>[3x]SKKLLFQFDTDATPSVFDVVVGYDGGADHITGYGNVTPDNVGAYVDGTIYTRGGKEKQSTAIFVGGGDMAAGERVFEAVKKRFFGPFRVSCMLDSNGSNTTAAAGVALVVKAAGGSVKGKKAVVLAGTGPVGMRSAALLAGEGAEVVLCGRKLDKAQAAADSVNKRFKVNVTAAETADDASRAEAVKGAHFVFTAGAI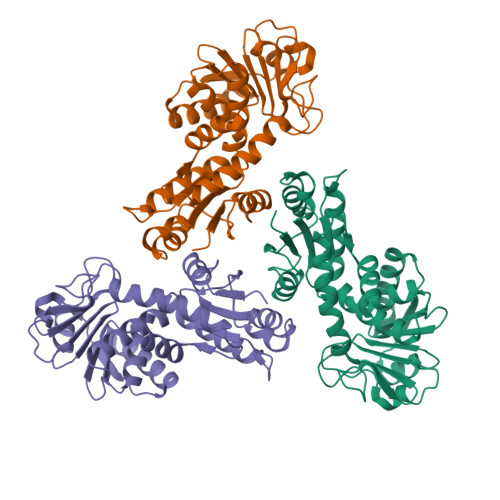GLELLPQAAWQNESSIEIVADYNAQPPLGIGGIDATDKGKEYGGKRAFGALGIGGLKLKLHRACIAKLFESSEGVFDAEEIYKLAKEMA>[12x]RRYMGSSHHHHHHMKLKIGITCYPSVGGSGVVGTELGKQLAERGHEIHFITSGLPFRLNKVYPNIYFHEVTVNQYSVFQYPPYDLALASKMAEVAQRENLDILHV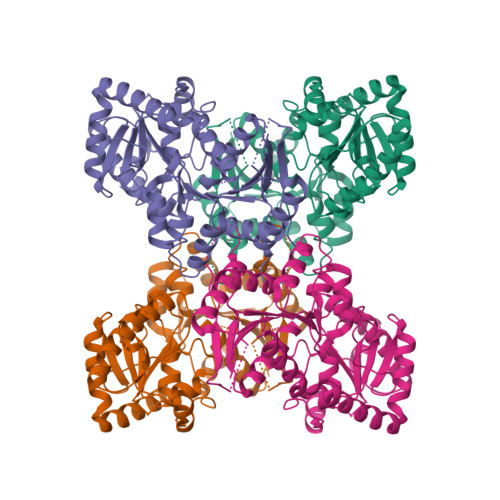HYAIPHAICAYLAKQMIGERIKIVTTLHGTDITVLGSDPSLNNLIRFGIEQSDVVTAVSHSLINETHELVKPNKDIQTVYNFIDERVYFKRDMTQLKKEYGISESEKILIHISNFRKVKRVQDVVQAFAKIVTEVDAKLLLVGDGPEFCTILQLVKNLHIEDRVLFLGKQDNVAELLAMSDLMLLLSEKESFGLVLLEAMACGVPCIGTRVGGIPEVIQHGDTGYLCEVGDTTGVADQAIQLLKDEELHRNMGERARESVYEQFRSEKIVSQYETIYYDVLRDDKNGKI>[6x]MLDSKLKAPVFTVRTQGREYGEFVLEPLERGFGVTLGNPLRRILLSSIPGTAVTSVYIEDVLHEFSTIPGVKEDVVEIILNLKELVVRFLNPSLQTVTLLLKAEGPKEVKARDFLPVADVEIMNPDLHIATLEEGGRLNMEVRVDRGVGYVPAEKHGIKDRINAIPVDAVFSPVRRVAFQVEDTRLGQRTDLDKLTLRIWTDGSVTPLEALNQAVEILREHLTYFSNPQAAAVAAPEEAKEPEAPPEQEEELDLPLEELGLSTRVLHSLKEEGIESVRALLALNLKDLKNIPGIGERSLEEIKEALEKKGFTLKE;>MEIKRFGRIREVIPLPPLTEIQVESYRRALQADVPPEKRENVGIQAAFRETFPIEEEDKGKGGLVLDFLEYRLGEPPFPQDECREKDLTYQAPLYARLQLIHKDTGLIKEDEVFLGHIPLMTEDGSFIINGADRVIVSQIHRSPGVYFTPDPARPGRYIASIIPLPKRGPWIDLEVEPNGVVSMKVNKRKFPLVLLLRVLGYDQETLARELGAYGELV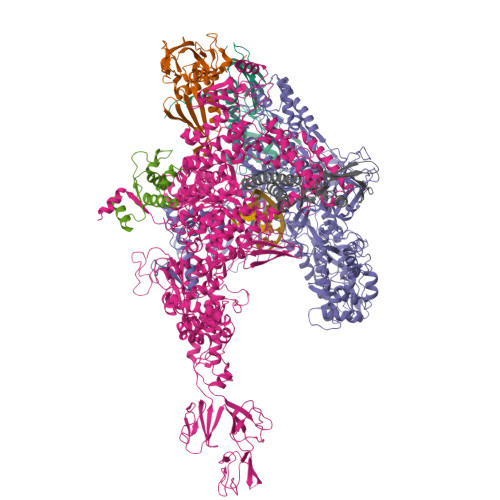QGLMDESVFAMRPEEALIRLFTLLRPGDPPKRDKAVAYVYGLIADPRRYDLGEAGRYKAEEKLGIRLSGRTLARFEDGEFKDEVFLPTLRYLFALTAGVPGHEVDDIDHLGNRRIRTVGELMTDQFRVGLARLARGVRERMLMGSEDSLTPAKLVNSRPLEAAIREFFSRSQLSQFKDETNPLSSLRHKRRISALGPGGLTRERAGFDVRDVHRTHYGRICPVETPEGANIGLITSLAAYARVDELGFIRTPYRRVVGGVVTDEVVYMTATEEDRYTIAQANTPLEGNRIAAERVVARRKGEPVIVSPEEVEFMDVSPKQVFSVNTNLIPFLEHDDANRALMGSNMQTQAVPLIRAQAPVVMTGLEERVVRDSLAALYAEEDGEVAKVDGNRIVVRYEDGRLVEYPLRRFYRSNQGTALDQRPRVVVGQRVRKGDLLADGPASENGFLALGQNVLVAIMPFDGYNFEDAIVISEELLKRDFYTSIHIERYEIEARDTKLGPERITRDIPHLSEAALRDLDEEGVVRIGAEVKPGDILVGRTSFKGESEPTPEERLLRSIFGEKARDVKDTSLRVPPGEGGIVVRTVRLRRGDPGVELKPGVREVVRVYVAQKRKLQVGDKLANRHGNKGVVAKILPVEDMPHLPDGTPVDVILNPLGVPSRMNLGQILETHLGLAGYFLGQRYISPIFDGAKEPEIKELLAQAFEVYFGKRKGEGFGVDKREVEVLRRAEKLGLVTPGKTPEEQLKELFLQGKVVLYDGRTGEPIEGPIVVGQMFIMKLYHMVEDKMHARSTGPYSLITQQPLGGKAQFGGQRFGEMEVWALEAYGAAHTLQEMLTLKSDDIEGRNAAYEAIIKGEDVPEPSVPESFRVLVKELQALALDVQTLDEKDNPVDIFEGLASKR[3x];>MKKEVRKVRIALASPEKIRSWSYGEVEKPETINYRTLKPERDGLFDERIFGPIKDYECACGKYKRQRFEGKVCERCGVEVTKSIVRRYRMGHIELATPAAHIWFVKDVPSKIGTLLDLSATELEQVLYFSKYIVLDPKGAILNGVPVEKRQLLTDEEYRELRYGKQETYPLPPGVDALVKDGEEVVKGQELAPGVVSRLDGVALYRFPRRVRVEYVKKERAGLRLPLAAWVEKEAYKPGEILAELPEPYLFRAEEEGVVELKELEEGAFLVLRREDEPVATYFLPVGMTPLVVHGEIVEKGQPLAEAKGLLRMPRQVRAAQVEAEEEGETVYLTLFLEWTEPKDYRVQPHMNVVVPEGARVEAGDKIVAAIDPEEEVIAEAEGVVHLHEPASILVVKARVYPFEDDVEVSTGDRVAPGDVLADGGKVKSDVYGRVEVDLVRNVVRVVESYDIDARMGAEAIQQLLKELDLEALEKELLEEMKHPSRARRAKARKRLEVVRAFLDSGNRPEWMILEAVPVLPPDLRPMVQVDGGRFATSDLNDLYRRLINRNNRLKKLLAQGAPEIIIRNEKRMLQEAVDALLDNGRRGAPVTNPGSDRPLRSLTDILSGKQGRFRQNLLGKRVDYSGRSVIVVGPQLKLHQCGLPKRMALELFKPFLLKKMEEKGIAPNVKAARRMLERQRDIKDEVWDALEEVIHGKVVLLNRAPTLHRLGIQAFQPVLVEGQSIQLHPLVCEAFNADFDGDQMAVHVPLSSFAQAEARIQMLSAHNLLSPASGEPLAKPSRDIILGLYYITQVRKEKKGAGLEFATPEEALAAHERGEVALNAPIKVAGRETSVGRLKYVFANPDEALLAVAHGIVDLQDVVTVRYMGKRLETSPGRILFARIVAEAVEDEKVAWELIQLDVPQEKNSLKDLVYQAFLRLGMEKTARLLDALKYYGFTFSTTSGITIGIDDAVIPEEKKQYLEEADRKLLQIEQAYEMGFLTDRERYDQILQLWTETTEKVTQAVFKNFEENYPFNPLYVMAQSGARGNPQQIRQLCGLRGLMQKPSGETFEVPVRSSFREGLTVLEYFISSHGARKGGADTALRTADSGYLTRKLVDVTHEIVVREADCGTTNYISVPLFQPDEVTRSLRLRKRADIEAGLYGRVLAREVEVLGVRLEEGRYLSMDDVHLLIKAAEAGEIQEVPVRSPLTCQTRYGVCQKCYGYDLSMARPVSIGEAVGIVAAQSIGEPGTQLTMRTFHTGGVAGAADITQGLPRVIELFEARRPKAKAVISEIDGVVRIEETEEKLSVFVESEGFSKEYKLPKEARLLVKDGDYVEAGQPLTRGAIDPHQLLEAKGPEAVERYLVEEIQKVYRAQGVKLHDKHIEIVVRQMMKYVEVTDPGDSRLLEGQVLEKWDVEALNERLIAEGKTPVAWKPLLMGVTKSALSTKSWLSAASFQNTTHVLTEAAIAGKKDELIGLKENVILGRLIPAGTGSDFVRFTQVVDQKTLKAIEEARKEAVEAKERPAARRGVKREQPGKQA[3x];>MAEPGIDKLFGMVDSKYRLTVVVAKRAQQLLRHGFKNTVLEPEERPKMQTLEGLFDDPNAVTWAMKELLTGRLVFGENLVPEDRLQKEMERLYPVEREE[3x];>MAREVKLTKAGYERLMQQLERERERLQEATKILQELMESSDDYDDSGLEAAKQEKARIEARIDSLEDILSRAVILEEGSGEVIGLGSVVELEDPLSGERLSVQVVSPAEANVLDTPMKISDASPMGKALLGHRVGDVLSLDTPKGRREFRVVAIHG[3x]> MLTEDQIKTTFADVAGCDEAKEEVAELVEYLREPSRFQKLGGKIPKGVLMVGPPGTGKTLLAKAIAGEAKVPFFTISGSDFVEMFVGVGASRVRDMFEQAKKAAPCIIFIDEIDAVGRQRGAGLGGGHDEREQTLNQMLVEMDGFEGNEGIIVIAATNRPDVLDPALLRPGRFDRQVVVGLPDVRGREQILKVHMRRVPLAPDIDAAIIARGTPGFSGADLANLVNEAALFAARGNKRVVSMVEFEKAKDK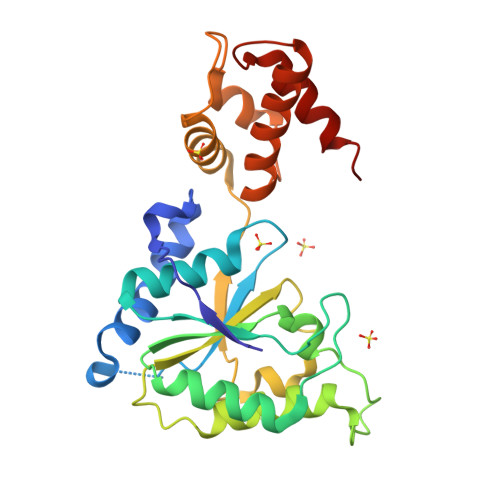IMMGLE>MGKTDQQVGAKLVQEIREGKRGPLYAGYFRTWHDRASTGIDGKQQHPENTMAEVPKEVDILFVFHDHTASDSPFWSELKDSYVHKLHQQGTALVQTIGVNELNGRTGLSKDYPDTPEGNKALAAAIVKAFVTDRGVDGLDIDIEHEFTNKRTPEEDARALNVFKEIAQLIGKNGSDKSKLLIMDTTLSVENNPIFKGIAEDLDYLLRQYYGSQGGEAEVDTINSDWNQYQNYIDASQFMIGFSFFEESASKGNLWFDVNEYDPNNPEKGKDIEGTRAKKYAEWQPSTGGL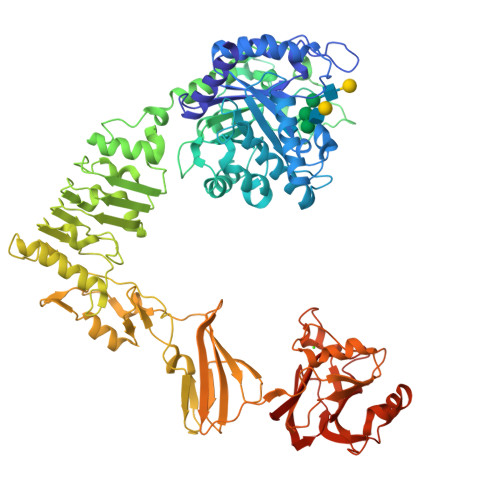KAGIFSYAIDRDGVAHVPSTYKNRTSTNLQRHEVDNISHTDYTVSRKLKTLMTEDKRYDVIDQKDIPDPALREQIIQQVGQYKGDLERYNKTLVLTGDKIQNLKGLEKLSKLQKLELRQLSNVKEITPELLPESMKKDAELVMVGMTGLEKLNLSGLNRQTLDGIDVNSITHLTSFDISHNSLDLSEKSEDRKLLMTLMEQVSNHQKITVKNTAFENQKPKGYYPQTYDTKEGHYDVDNAEHDILTDFVFGTVTKRNTFIGDEEAFAIYKEGAVDGRQYVSKDYTYEAFRKDYKGYKVHLTASNLGETVTSKVTATTDETYLVDVSDGEKVVHHMKLNIGSGAIMMENLAKGAKVIGTSGDFEQAKKIFDGEKSDRFFTWGQTNWIAFDLGEINLAKEWRLFNAETNTEIKTDSSLNVAKGRLQILKDTTIDLEKMDIKNRKEYLSNDENWTDVAQMDDAKAIFNSKLSNVLSRYWRFCVDGGASSYYPQYTELQILGQRLSNDVANTLKDL[2x]> 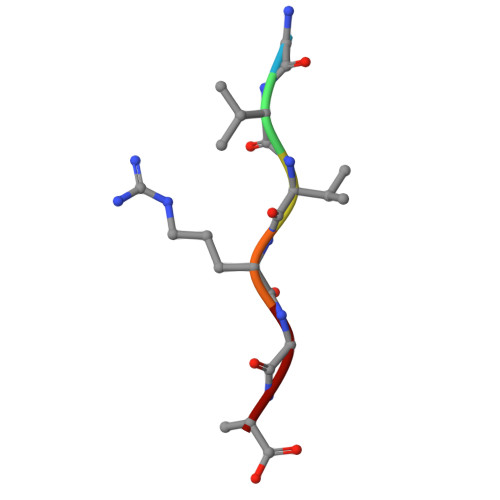GVVRGA> PPPVGP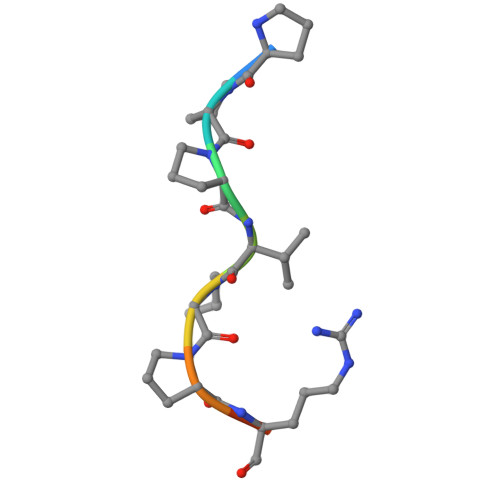RRR>MHHHHHHHHHHHHLPPITPQELESMSPQEQRAALGDRLFLKVYEIAPELAPKITGMFLEMKPKE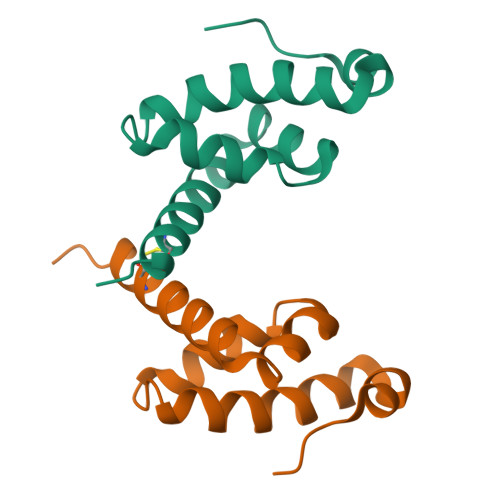AYELLNDQKRLEERVTEALCVLKAHQTA[2x]> A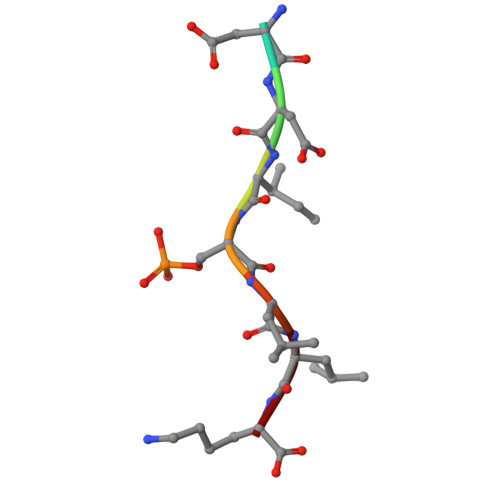DDISLLK>[13x]MAFLGAAIAAGLAAVAGAIAVAIIVKATIEGTTRQPELRGTLQ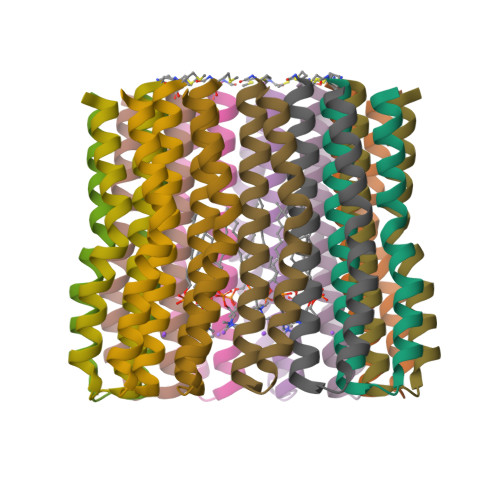TLMFIGVPLAEAVPIIAIVISLLILF>[2x]TFDVGDEYEIIETIGNGAYGVVSSRRRRLTGQQVAIKKIPNAFDVVTNAKRTLRELKILKHFKHDNII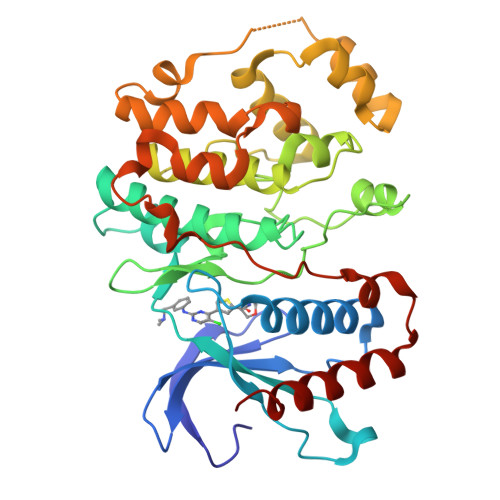AIKDILRPTVPYGEFKSVYVVLDLMESDLHQIIHSSQPLTLEHVRYFLYQLLRGLKYMHSAQVIHRDLKPSNLLVNENCELKIGDFGMARGLCTSPAEHQYFMTEYVATRWYRAPELMLSLHEYTQAIDLWSVGCIFGEMLARRQLFPGKNYVHQLQLIMMVLGTPSPAVIQAVGAERVRAYIQSLPPRQPVPWETVYPGADRQALSLLGRMLRFEPSARISAAAALRHPFLAKYHDPDDEPDCAPPFDFAFDREALTRERIKEAIVAEIEDFHARRE> GGIGENEWVKILR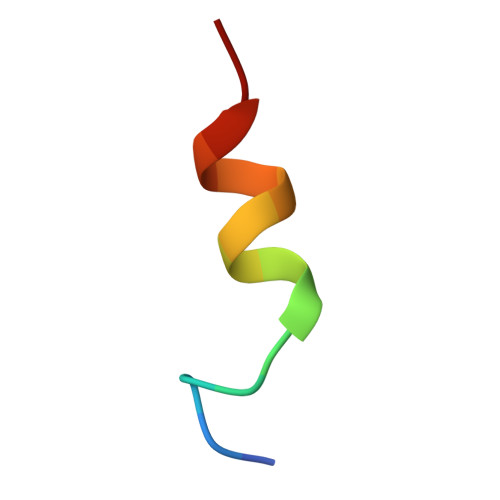SKR> GSHMSSLPVPYKLPVSLSVGSCVIIKGTPIHSFINDPQLQVDFYTD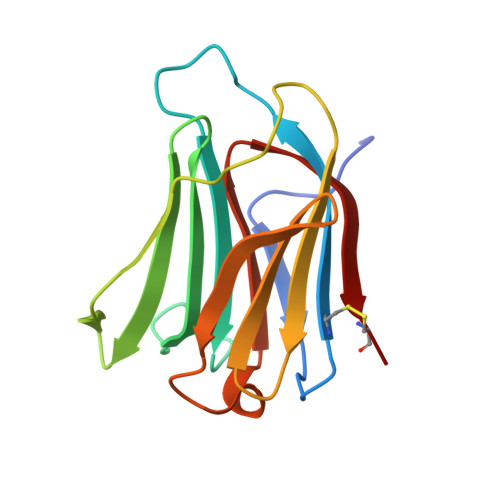MDEDSDIAFRFRVHFGNHVVMNRREFGIWMLEETTDYVPFEDGKQFELCIYVHYNEYEIKVNGIRIYGFVHRIPPSFVKMVQVSRDISLTSVSVCN4-methoxybenzenesulfonamide | 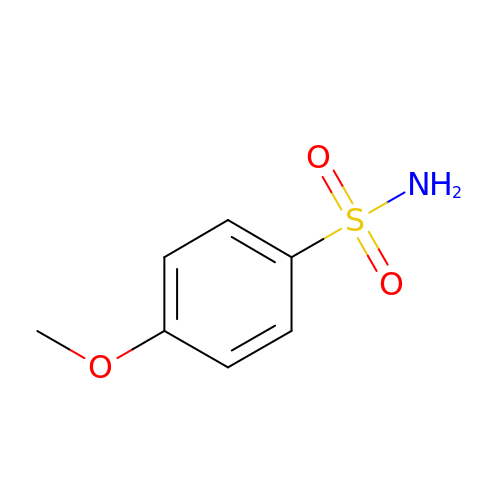C7 H9 N O3 S | MSFQEZBRFPAFEX-UHFFFAOYSA-N> MSLLKMLDKLSLESIEDQGTTIHGDVELVVENETSADVSSVLAEVDQIENNPVEEVLDADDAVQPTALDTEVTIVQAEDELGLIEDAKEALEKFQGLLLQAGEDGISRQAAAFMHVGMESIDRILGIEKSGLTAALENYDASPRSAIQKAAVISLEDLKEKLKEAGKKALEIIKKIVAMIKQKIKDFNPKLIALDMRITKTIDAIKSLKAGDLKKEEIKFTPSEY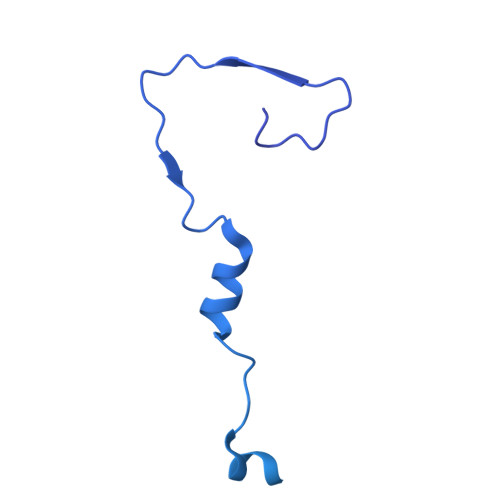MVSSSGFIANNPKTIADFMTVFSTQYVSALRKYGELGVRYLKGDKSIDIDQVTSDLQAKMAEDINKAVEKAPGNVKLEVTSSKSGVNKWEVVEGDGETDLHEVEVDVRAPSKILAHLNILKGLVIKLQDFNKIDYKIAENLEKALADWNPDEAGMSKETARDALNIGGIDNSALVNYIAKCIAAQYTFIVKHELAAYGKETSKAPENDEK> LSKHTTTLYEIIESELQRLGLNEFVNNDRIHFNDSKHAFMQKMLYFDDDVKQIVDHMFFKGFMFNDERIDRYFKESFTLRFLYREIGRQTVESFASQVLYI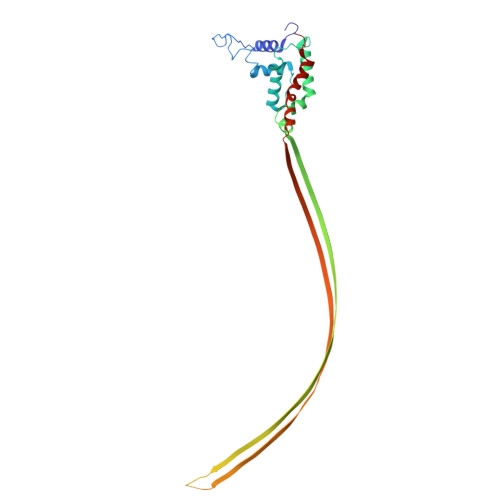TMTHEDYIYRVYGSDMYKYIEQVTDTQSQDLGKAIENAIEQGQTKDRQQDKGHEEYKDYEDTITKSFDDNRTAESTLPQSKVNIDVDNTVLDYADTNTISRDKNTSETVSEKTGTKDNTFDSLRNGESDTKRNTQSQNEMNRTGLTKQYLIDNLQKLYSMRDTIFKTYDKECFLHIW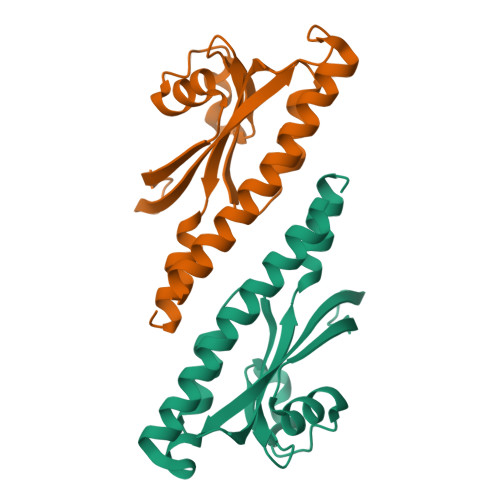>[2x]MNNLEKELLDNFKKNITQYAKQLEISIEKVYDEKGSVNAQKDIQNLLSEYANCQEIGEIRFIDKDQIIIATTKQSNRSLINQKANDSSVQKALSLGQSNDHLILKDYGGGKDRVWVYNIPVKVDKKVIGNIYIESKINDVYNQLNNINQ> GPACPTHADSLNNLANIKREQGNIEEAVRLYRKALE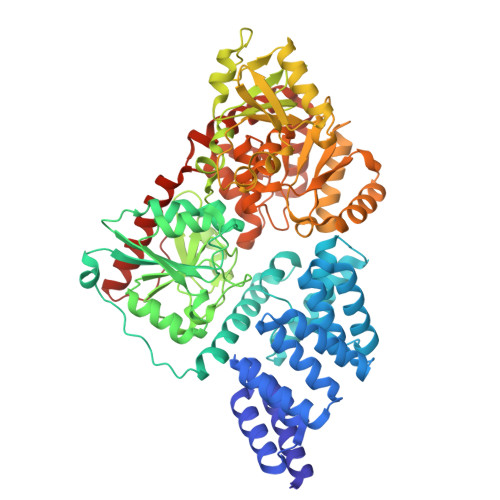VFPEFAAAHSNLASVLQQQGKLQEALMHYKEAIRISPTFADAYSNMGNTLKEMQDVQGALQCYTRAIQINPAFADAHSNLASIHKDSGNIPEAIASYRTALKLKPDFPDAYCNLAHCLQIVCDWTDYDERMKKLVSIVADQLEKNRLPSVHPHHSMLYPLSHGFRKAIAERHGNLCLDKINVLHKPPYEHPKDLKLSDGRLRVGYVSSDFGNHPTSHLMQSIPGMHNPDKFEVFCYALSPDDGTNFRVKVMAEANHFIDLSQIPCNGKAADRIHQDGIHILVNMNGYTKGARNELFALRPAPIQAMWLGYPGTSGALFMDYIITDQETSPAEVAEQYSEKLAYMPHTFFIGDHANMFPHLKKKAVIDFKSNGHIYDNRIVLNGIDLKAFLDSLPDVKIVKMKCPDGGDNADSSNTALNMPVIPMNTIAEAVIEMINRGQIQITINGFSISNGLATTQINNKAATGEEVPRTIIVTTRSQYGLPEDAIVYCNFNQLYKIDPSTLQMWANILKRVPNSVLWLLRFPAVGEPNIQQYAQNMGLPQNRIIFSPVAPKEEHVRRGQLADVCLDTPLCNGHTTGMDVLWAGTPMVTMPGETLASRVAASQLTCLGCLELIAKNRQEYEDIAVKLGTDLEYLKKVRGKVWKQRISSPLFNTKQYTMELERLYLQMWEHYAAGNKPDHMIKPVEVTESA> MASSCAVQVKLELGHRAQVRKKPTVEGFTHDWMVFVRGPEHSNIQHFVEKVVFHLHESFPRPKRVCKDPPYKVEESGYAGFILPIEVYFKNKEEPRKVRFDYDLFLHLEGHPPVNHLRCEKLTFNNPTEDFRRKLLKA

Recently, the YEATS (YAF9, ENL, AF9, TAF14, SAS5) domains were identified as “readers” of lysine acylation, including acetylation and crotonylation. Unlike the bromodomains with end-closed binding cavities, the YEATS domain adopts an end-open aromatic “sandwich” cage to recognize histone lysine acylation. The AF9 YEATS domain adopted an immunoglobin fold that consisted of a two-layer β sandwich between eight antiparallel β strands. The AF9/ENL YEATS domains recognize acylated histones to recruit the super elongation complex and, in turn, DOT1L on active chromatin.

As the crystal structure also revealed that the methoxyl group of hit 2 pointed toward the unoccupied groove surrounded by residues F28, P60, and E75, we substituted the methyl group with a benzyl or phenyl group (compounds 10 and 11). Compound 10 achieved an approximately two-fold enhancement of the affinity for the AF9 YEATS domain. We hence solved the crystal structure of the AF9 YEATS domain in complex with compound 10 with clear electron density, diffracted at 1.8 Å. In general, compounds 2 and 10 demonstrated a conserved pose and thus shared a similar interaction pattern. However, compound 10 bound deeper along the same aromatic groove and thus had a more intimate cavity encapsulation than compound 2 did. Therefore, the benzyl substituent of compound 10 had additional interactions with residues P60 and F28 for enhanced affinity to AF9 YEATS. Sequence alignment of the AF9/ENL YEATS domains suggested a conserved aromatic cage in AF9 and ENL. It is, therefore, difficult to achieve a high selectivity between AF9 and ENL YEATS domains, as underscored by the similar affinity of compound 10 to both AF9 and ENL (38 ± 6 μM) determined by CSPs, even though compound 10 represented a new chemotype with a binding mode distinct from that of SGC-iMLLT. Therefore, compound 10 was a dual inhibitor of AF9/ENL YEATS domains. Compound 10 had weak potency in MCF7 cells using a Cell Counting Kit-8 (CCK-8) assay, but suppressed the proliferation of AF9-sensitive HGC-27 cells more effectively in a dose-dependent manner, which is consistent with the CRISPR result. Inhibitors harboring the new chemotypes were then uncovered guided by complex crystal structures, which revealed a binding mode to form an extra hydrogen bond in comparison with SGC-iMLLT.> GMYGKGKSNSSAVPSDSQAREKLALYVYEYLLHVGAQKSAQTFLSEIRWEKNITLGEPPGFLHSWWCVFWDLY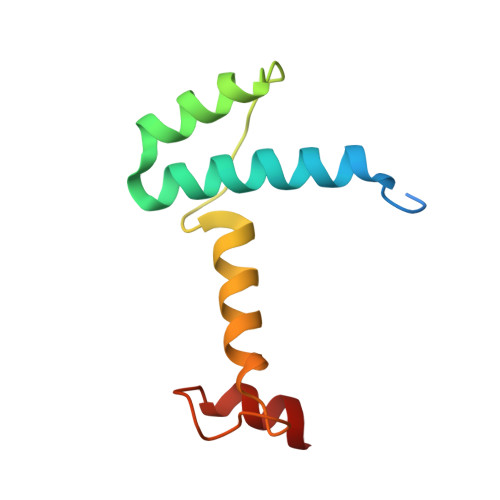CAAPERRETCEHSSEAKAFHDY> DEEITCQENNPFTCGNTDGLNSSSFEADFIFGVASSAYQIEGTIGRGLNIWDGFTHRYPDKSGPDHGNGDTTCDSFSYWQKDIDVLDELNATGYRFSIAWSRIIPRGKRSRGVNQKG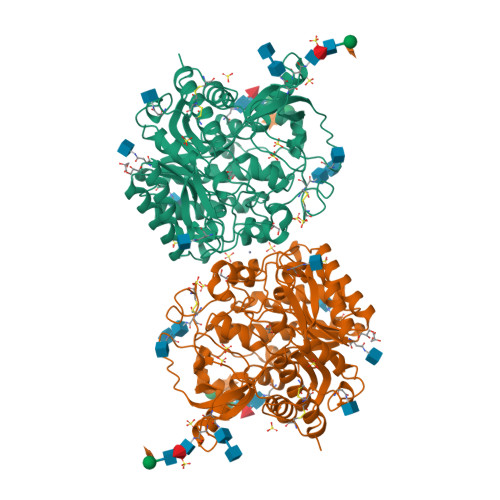IDYYHGLIDGLIKKGITPFVTLFHWDLPQTLQDEYEGFLDPQIIDDFKDYADLCFEEFGDSVKYWLTINQLYSVPTRGYGSALDAPGRCSPTVDPSCYAGNSSTEPYIVAHHQLLAHAKVVDLYRKNYTHQGGKIGPTMITRWFLPYNDTDRHSIAATERMKQFFLGWFMGPLTNGTYPQIMIDTVGARLPTFSPEETNLVKGSYDFLGLNYYFTQYAQPSPNPVNATNHTAMMDAGAKLTYINASGHYIGPLFESDGGDGSSNIYYYPKGIYSVMDYFKNKYYNPLIYVTENGISTPGSENRKESMLDYTRIDYLCSHLCFLNKVIKEKDVNVKGYLAWALGDNYEFNNGFTVRFGLSYINWNNVTDRDLKKSGQWYQKFISP>SEYCSHMIGSGHLQSLQRLIDSQMETSCQITFEFVDQEQLKDPVCYLKKAFLLVQDIMEDTMRFRDNTPNAIAIVQLQELSLRLKSCFTKDYEEHDKACVRTFYETPLQLLEKVKNVFNETKNLLDKDWNIFSKNCNNSFAECSSQGH[2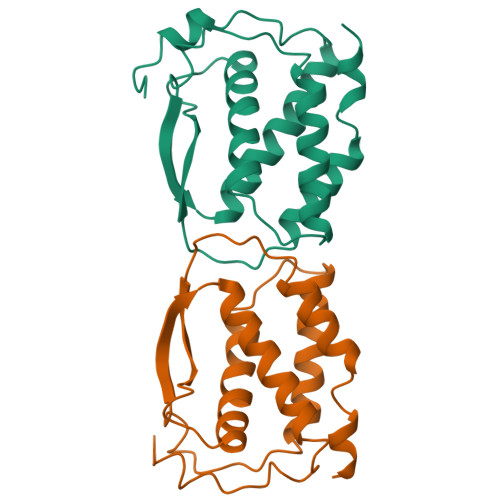x]1-(4-CARBOXY-2-GUANIDINOPENTYL)-5,5'-DI(HYDROXYMETHYL)PYRROLIDIN-2-ONE | C14 H18 N4 O5 | 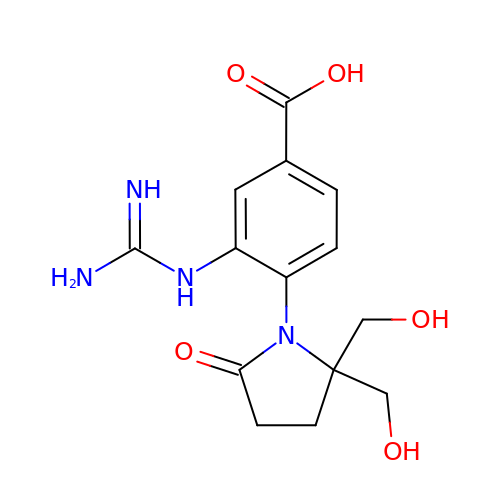IRNYFKBSAARAHR-UHFFFAOYSA-N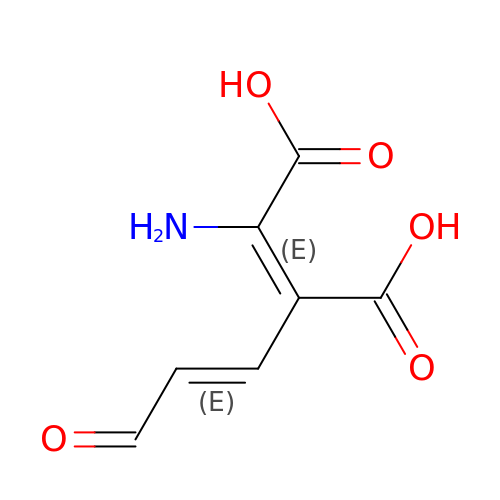(2E)-2-amino-3-[(1E)-3-oxoprop-1-en-1-yl]but-2-enedioic acid | C7 H7 N O5 | KACPVQQHDVBVFC-PMRVSPHWSA-N>[4x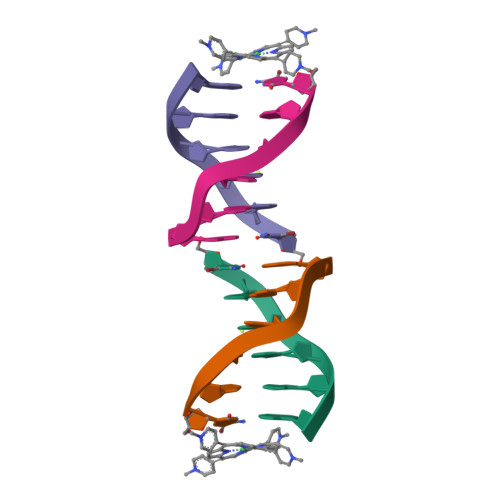]CCTAGG Structural analyses of two glycoside hydrolase family 92 α-mannosidases, BT3130 and BT3965, together with mechanistically relevant complexes at 1.8–2.5 Å resolution reveal conservation of the global enzyme fold and core catalytic apparatus despite different linkage specificities. Most enzymes within family GH92 are exo-acting α-mannosidases that are capable of hydrolysing terminal mannosidic residues with a variety of linkages, including α-1,2, α-1,3, α-1,4 and α-1,6 glycosidic bonds. Complementary to α-mannosidases within largely eukaryotic mannosidase families (particularly GH38 and GH47) that play important roles in N-glycan processing, GH92 enzymes are metal-dependent, featuring a single Ca2+ ion coordinated within the catalytic active site. GH92 enzymes act via a classic single-displacement mechanism, leading to inverted configuration at the anomeric centre.

The three-dimensional structures of BT3130 and BT3965 both reveal a two-domain enzyme that appears to be well conserved with published examples of GH92 α-mannosidases. Indeed, quantitative structural comparison using the DALI server shows that the three-dimensional structures of BT3130 and BT3965 have high similarity, with an r.m.s.d. of 1.4 Å mapped over 738 matched Cα positions (sequence identity = 40%, Z-score = 48.7). Like the members of the exo-α-mannosidase families GH38 and GH47, GH92 enzymes are metal-dependent, and a single calcium ion is observed coordinated within the active sites of both BT3130 and BT3965. Interestingly, however, while Ca2+ derived from the bacterial expression host was consistently observed within previous structures of BT3990, both BT3130 and BT3965 showed a somewhat reduced ability to bind and sequester this required divalent cation. Therefore, to ensure observation of the true, catalytically competent forms of these enzymes, and the determination of meaningful ligand complexes, BT3130 was screened for crystallization with the addition of 10 mM calcium acetate (final concentation) to the protein buffer (in addition to avoiding K+-containing screen hits), while the subsequent ManI complexes of both enzymes were cryoprotected with the addition of 1 mM Ca2+ (final concentration) to the cryoprotectant solutions. Within BT3130, the 580-loop is positioned lower, and projects into the +1 subsite at a steeper angle, leaving a larger solvent-exposed space at the outer surface of the substrate-binding cavity. Furthermore, the hydrophobic ‘roof’ of this subsite is contributed by Trp67 (rather than Trp88 as in BT3990) and appears shifted some 2.5 Å towards the outer surface. BT3130 and BT3965 are found together within the same clade, and are distinct from previously published structures of the α-1,2-specific enzymes BT3990 and BT2199.

>MGQAGEITKYVNPFIGTGAIDGGLSGNNYPGATSPFGMIQLSPDTSEAPNWGDASGYDYNRNTIFGFSHTRLSGTGASDLIDITLMPTSSGRTSSAFTHDEEKARPGYYQVMLKDENINAELTTTQRNGIHRYQYPAGKDAEIILDMDHSADKGSWGRRIINSQIRILNDHAVEGYRIITGWAKLRKIYFYMEFSSPILTSTLRDGGRVHENTAVINGTNLHGCFRFGQLNGKPLTCKVALSSVSMENARQNMEQEAPHWDFDRYVAAADADWEKQLGKIEVKGTEVQKEIFYTALYHTMIQPNTMSDVNGEYMAADYTTRKVANNETHYTTFSLWDTFRASHPLYTLLEPERVTDFVKSMIRQYEYYGYLPIWQLWGQDNYCMIGNHSIPVITDAILKGIPGIDMEKAYEAVYNSSVTSHPNSPFEVWEKYGFMPENIQTQSVSITLEQAFDDWCVAQLAAKLNKDADYQRFHKRSEYYRNLFHPKTKFFQSKNDKGEWIEPFDPYQYGGNGGHPFTEGNAWQYFWYVPHNIQALMELTGGTKAFEQKLDTFFTSTYKSEQMNHNASGFVGQYAHGNEPSHHVAYLYNFAGQPWKTQKYVSHILNTLYNNTSSGYAGNDDCGQMSAWYVFSAMGFYPVNPADGRYIIGSPLLDECTLKLAGNKEFRIRTIRKSPEDIYIQSVTLNGKKHKDFFITHQDIMNGGTMVFKMGKKPSGWGKLEHHHHHH[3x]> SHNEKLAKKKIVSIDAGRKYFSPEQLKEIIDKAKHYGYTDLHLLVGNDGLRFMLDDMSITANGKTYASDDVKRAIEKGTNDYYNDPNGNHLTESQMTDLINYAKDKGIGLIPTVNSPGHMDAILNAMKELGIQNPNFSYFGKKSARTVDLDNEQAVAFTKALIDKYAAYFAKKTEIFNIGLDEYANDATDAKGWSVLQADKYYPNEGYPVKGYEKFIAYANDLARIVKSHGLKPMAFNDGIYYNSDTSFGSFDKDIIVSMWTGGWGGYDVASSKLLAEKGHQILNTNDAWYYVLGRNADG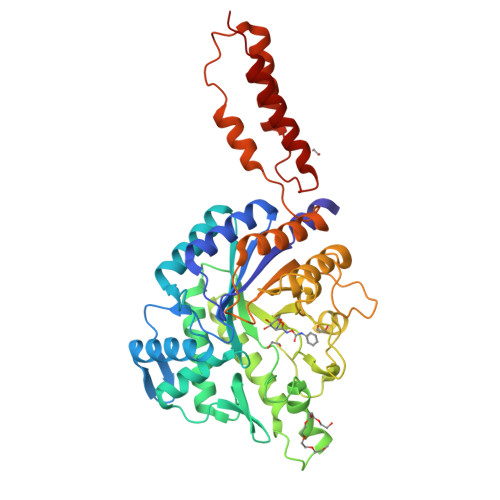QGWYNLDQGLNGIKNTPITSVPKTEGADIPIIGGMVAAWADTPSARYSPSRLFKLMRHFANANAEYFAADYESAEQALNEVPKDLNRYTAESVTAVKEAEKAIRSLDSNLSRAQQDTIDQAIAKLQETVNNLTLT>MKHHHHHHSAGLEVLFQGPRRQTIEALVPAWDSDIIFKCLCYFHTLYPGLIPLETFPPATIFNFKQKIISILEDKKAVLRGEPIKGPLPICCSKENYRRHLQRTTLLPVFMWYHPTPKTLSDTMQTMKQLAIKGSVGASHWLLVIVDIQARRLVYFDSLYNYVMPPENMKKELQSFAQQLDQVYPAYDSKKFSVKIAAKEVIQRGSGSSCGAWCCQFLHWYLKDPLTDALNDLPVDSVERHENLASFVQACEAAVQDL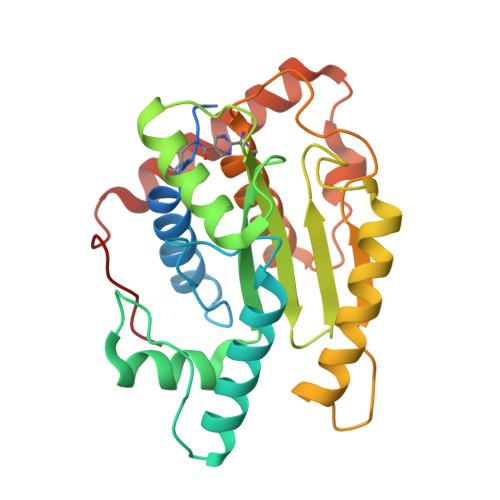PELSWPEA[2x]>MSSLNQLVSGLASGAVRIVDLTHTLDPDFPVIVLPPEFGQCARFRMEEISAYDHRGPAWKWHNISMSEHTGTHFDAPSHWI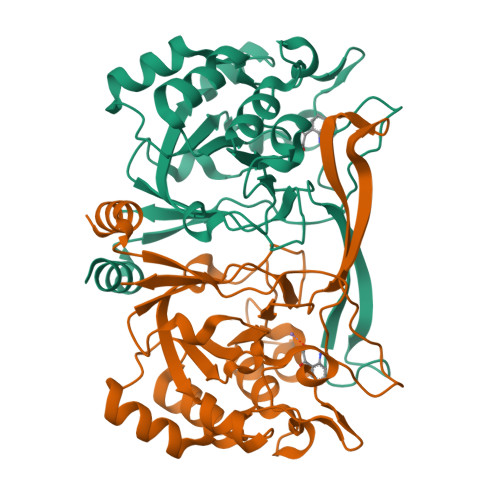SGKDVPNGSVDEIPAEAFVGPVVVIDCSKGAAENDDFELTPEIIAGWESEHGRIPEDAWVLMRTDWSKRRGADYLNMRADGPHSPGPTPEAIRFLIEERNIRGFGTETVGTDAGQGAHYVPPYPAHYLLHGAGKYGLQCLANLDQLPATGAVLIAAPLKIKNGTGSPLRVLAMVTE[4x]>[2x]AAAAAACUUACUAUUAUAUUUGUAACAAAUUUUAUACAUAAGAUAAAUUCGUAUGUAUAGCCGUUCUGCUCGA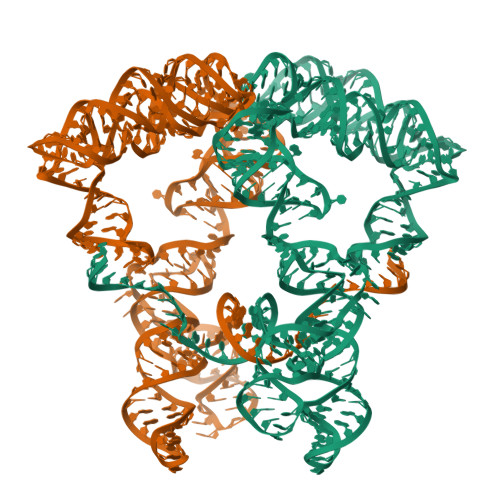AACGGUAUAGCACCGUAAUGGUGGUAUUAUGAAUUGUAGCAAGGUGCGAGGCUACCUUUAAAAGUCUUGGAGGUGCUCUGAGUGGGUACUUUAUUAGGGUUAUAAUUUAGAAAGUAAGCUAAAACUCUAGGUGUUGGGCAGGGCUAACACUGGCAUAUAAUUAAAUAUGCGAUAAAGUAAGU Recently, RNF112 has emerged as an intriguing addition to the dynamin-like large GTPase superfamily, which has been widely implicated in mediating biological membrane remodeling events, including membrane tubulation, fission, and fusion. To obtain an architectural overview of RNF112, we carried out structural studies on modified Xenopus laevis RNF112 constructs in different nucleotide-loading states. For these constructs (collectively denoted as RNF112T), the N-terminal RING domain, the predicted transmembrane helix, and the C-terminal amphipathic helix were removed. RNF112T is composed of a GTPase domain (GD) and a middle domain (MD) comprising a 3-helix bundle.

We also determined another GDP-bound RNF112T structure derived from a nucleotide-free RNF112T crystal soaked with GDP (RNF112T-GDP form 2). In this structure, parts of G2/switch I and G3/switch II are disordered, whereas the G1/P-loop and G4 mediating the GDP molecule become discernable compared to the nucleotide-free structure. Interestingly, Arg195 of RNF112T-GDP form 1, but not of RNF112T-GDP form 2, adopts a conformation consistent with that of the RNF112T-GDP•AlF4− complex at the catalytic site, and maintains the same hydrogens bonds with residues from G2/switch I. However, nucleotide-free RNF112T and RNF112T-GDP form 2 adopt a unique conformation that has never been observed with ATLs.

>[2x]AEPDHPIQLVWTDVNGRLSLDLSGAHDCFLNTRYSNYPVFILCIIGEKRRGKSFLMNYIMRALRSMEMDEEISLGADDEPLKGFKWSPGTETTTKGIWMWNRPFLLNHKGGKIAVFLLDTEGSLDIESDRETCIKLSALSLFISSHLIFNVASNLKETELDYMEMYMNMGEECGPKNLQHLDILVRDWYHSKKWDRDVARSYISREIEKLEKLNSYPKVLWSLKSNQTRCFLLPHPGKGITGESEGRLQDMDEDFQESLRSYVSKVVKGICTHIKTNIDGELLTSAHVFSMLQEFTEVLNLQIYGFSSPMEMFYAIKNQKLMGEIENEFQDFLKNQSSLTLPPTMRVKVSQKFSELLEKFMQFVQGSNTSSHDAMLKDLEVRLLEIQEKFCNDFTTRFT(2S)-2-(4-chlorobenzyl)-3-oxo-3-[4-(7H-pyrrolo[2,3-d]pyrimidin-4-yl)piperazin-1-yl]propan-1-amine | C20 H23 Cl N6 O | 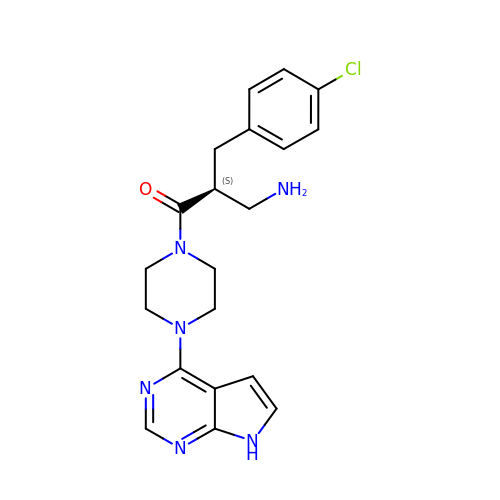IYQSFRNHWXBIKV-HNNXBMFYSA-N>SHAPTRSARDIHQLEARIDSLAARNSKLMETLKEARQQLLALREEVDRLGQ[2x];>STAAGQERREKLTEETDDLLDEIDDVLEENAEDFVRAY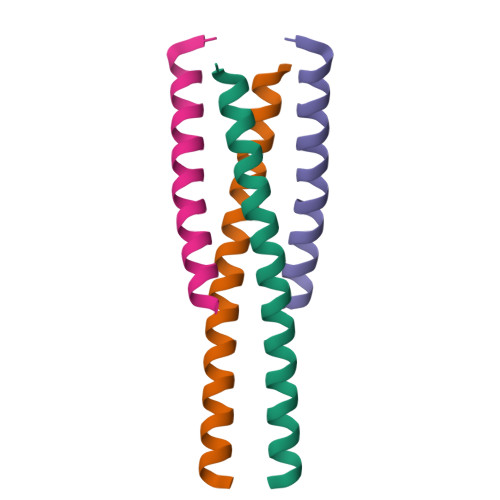VQKGGE[2x]>[2x]MKQYLELMQKVLDE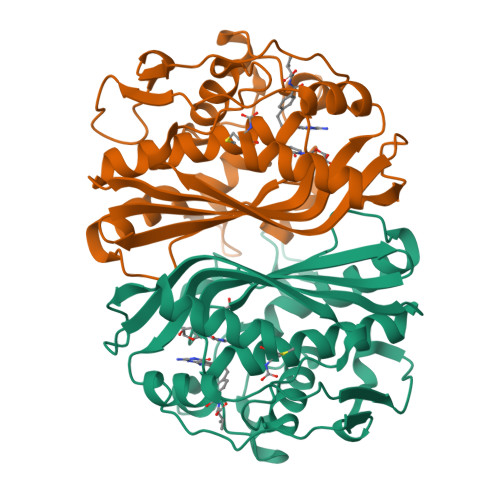GTQKNDRTGTGTLSIFGHQMRFNLQDGFPLVTTKRCHLRSIIHELLWFLQGDTNIAYLHENNVTIWDEWADENGDLGPVYGKQWRAWPTPDGRHIDQITTVLNQLKNDPDSRRIIVSAWNVGELDKMALAPCHAFFQFYVADGKLSCQLYQRSCDVFLGLPFNIASYALLVHMMAQQCDLEVGDFVWTGGDTHLYSNHMDQTHLQLSREPRPLPKLIIKRKPESIFDYRFEDFEIEGYDPHPGIKAPVAI>MGHHHHHHYVDRKPSLYLEDLRHDFKNSLSKFENGDEAFDTLLGFVELDHIYSSALKEISTKLSILDDNFNHIYKHNPIHHMERRVKEMRSLIEKLNRKGLQISAETAKEHILDIAGIRVVCNYLDDIYLIEEMLLKQEDVQLIKRKDYIQHPKENGYRSLHIVVSIPVFLAERVEVLPVEIQIRTIGMDMWASLEHKIRYKNNAETEKY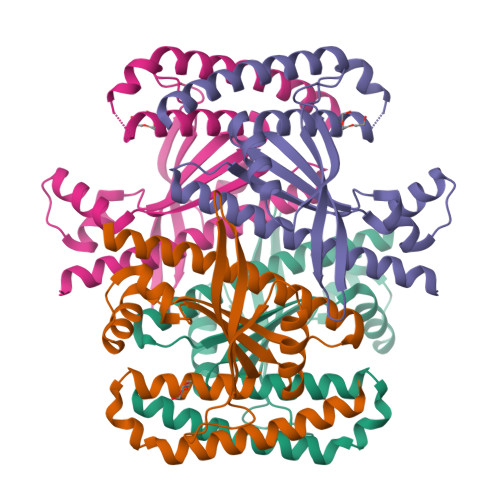RDLLKECATEITEVEDKLQQIHSEITE[2x]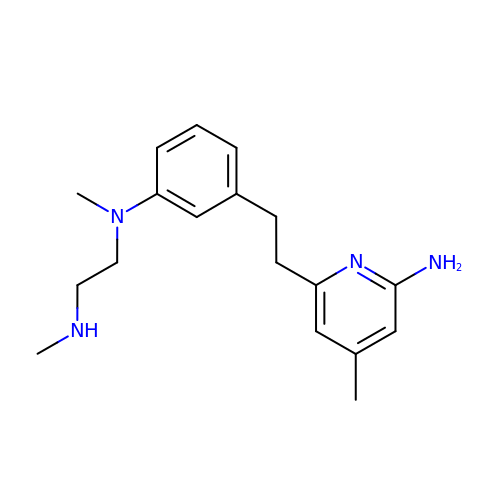N1-(3-(2-(6-Amino-4-methylpyridin-2-yl)ethyl)phenyl)-N1,N2-dimethylethane-1,2-diamine | C18 H26 N4 | MIKRWQRFDGLBCF-UHFFFAOYSA-N> MAQNPFKALNINIDKIESALTQNGVTNYSSNVKNERETHISGTYKGIDFLIKLMPSGGNTTIGRASGQNNTYFDEIALIIKENCLYSDTKNFEYTIPKFSDDDRANLFEFLSEE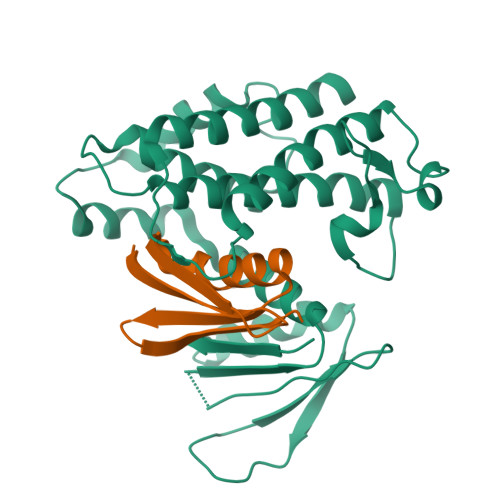GITITEDNNNDPNCKHQYIMTTSNGDRVRAKIYKRGSIQFQGKYLQIASLINDFMCSILNMKEIVEQKNKEFNVDIKKETIESELHSKLPKSIDKIHEDIKKQLSCSLIMKKIDVEMEDYSTYCFSALRAIEGFIYQILNDVCNPSSSKNLGEYFTENKPKYIIREIHQETINGEIAEVLCECYTYWHENRHGLFHMKPGIADTKTINKLESIAIIDTVCQLIDGGVARLKL;> MELVKVVFMGWFKNESMFTKEITMMKDDVQWATTQYAEVNKALVKAFIDDKKVCEVDCRG Here, we present several cryo-EM structures of the mitochondrial RNase Z complex (ELAC2/SDR5C1/TRMT10C) bound to different maturation states of mitochondrial tRNAHis, showing the molecular basis for tRNA-substrate selection and catalysis. The human long form of RNase Z, ELAC2, has two alternative start codons to produce a nuclear and a mitochondrially targeted form. TRMT10C is a purine N1-methyltransferase that acts at position 9 of mt-tRNAs using S-adenosylmethionine (SAM) as a co-substrate. SDR5C1 is a moonlighting homotetrameric short-chain dehydrogenase/reductase.

The reconstituted catalytically active RNase Z was incubated to complete turnover and used to determine a cryo-EM structure of the ternary product complex of human RNase Z to an overall resolution of 2.9 Å. In our product complex RNase Z-HS, the discriminator base C73 is positioned in the active site, with its ribose-O3 in the expected position directly after catalysis. Furthermore, the C73 backbone phosphate is wedged between S490, S768, and K700, whereas R728 in the conserved 724-HFSQRY-729 motif clamps the C72 and C73 backbone phosphates. In the mitochondrial RNase Z complex, ELAC2 binds to the mt-tRNA T loop and the TRMT10C N-terminal domain through the exosite. The exosite establishes electrostatic interactions with the T loop backbone U55 via K279 and N253. The ELAC2 C-terminal α-helix (α25), which is only present in long-form homologs, contributes further to mitochondrial RNase Z complex formation. The C-terminal helix contains R788, which interacts with the backbone of U69, located close to the tip of the acceptor stem. The C-terminal α helix sterically hinders a 5′-extension of the mt-tRNA (Fig. EV2C) and, therefore, provides the structural basis for the 5′-to-3′ processing order observed in vivo and in vitro. In addition, ELAC2 residues R381, K495, and K731 interact with the 5′-α-phosphate of the mt-tRNAHis.

>[4x]MAAACRSVKGLVAVITGGASGLGLATAERLVGQGASAVLLDLPNSGGEAQAKKLGNNCVFAPADVTSEKDVQTALALAKGKFGRVDVAVNCAGIAVASKTYNLKKGQTHTLEDFQRVLDVNLMGTFNVIRLVAGEMGQNEPDQGGQRGVIINTASVAAFEGQVGQAAYSASKGGIVGMTLPIARDLAPIGIRVMTIAPGLFGTPLLTSLPEKVCNFLASQVPFPSRLGDPAEYAHLVQAIIENPFLNGEVIRLDGAIRMQP;> SRPRKDPLRHLRTREKRGPSGCSGGPNTVYLQVVAAGSRDSGAALYVFSEFNRYLFNCGEGVQRLMQEHKLKVARLDNIFLTRMHWSNVGGLSGMILTLKETGLPKCVLSGPPQLEKYLEAIKIFSGPLKGIELAVRPHSAPEYEDETMTVYQIPIHSEQRRGKHQPWQSPERPLSRLSPERSSDSESNENEPHLPHGVSQRRGVRDSSLVVAFICKLHLKRGNFLVLKAKEMGLPVGTAAIAPIIAAVKDGKSITHEGREILAEELCTPPDPGAAFVVVECPDESFIQPICENATFQRYQGKADAPVALVVHMAPASVLVDSRYQQWMERFGPDTQHLVLNENCASVHNLRSHKIQTQLNLIHPDIFPLLTSFRCKKEGPTLSVPMVQGECLLKYQLRPRREWQRDAIITCNPEEFIVEALQLPNFQQSVQEYRRSAQDGPAPAEKRSQYPEIIFLGTGSAIPMKIRNVSATLVNISPDTSLLLDCGEGTFGQLCRHYGDQVDRVLGTLAAVFVSHLHADHHTGLPSILLQRERALASLGKPLHPLLVVAPNQLKAWLQQYHNQCQEVLHHISMIPAKCLQEGAEISSPAVERLISSLLRTCDLEEFQTCLVRHCKHAFGCALVHTSGWKVVYSGDTMPCEALVRMGKDATLLIHEATLEDGLEEEAVEKTHSTTSQAISVGMRMNAEFIMLNHFSQRYAKVPLFSPNFSEKVGVAFDHMKVCFGDFPTMPKLIPPLKALFAGDIEEMEERREKRELRQVRAALLSRELAGGLEDGEPQQKRAHTEEPQAKKVRAQ;> MKSSVQEECVSTISSSKDEDPLAATREFIEMWRLLGREVPEHITEEELKTLMECVSNTAKKKYLKYLYTKEKVKKARQIKKEMKAAAREEAKNIKLLETTEEDKQKNFLFLRLWDRNMDIAMGWKGAQAMQFGQPLVFDMAYENYMKRKELQNTVSQLLESEGWNRRNVDPFHIYFCNLKIDGALHRELVKRYQEKWDKLLLTSTEKSHVDLFPKDSIIYLTADSPNVMTTFRHDKVYVIGSFVDKSMQPGTSLAKAKRLNLATECLPLDKYLQWEIGNKNLTLDQMIRILLCLKNNGNWQEALQFVPKRKHTGFLEISQHSQEFINRLKKAKTAENLYFQSHHHHHHDYKDDDDK>[2x]GSSSTEVKDNVLTEEEKAEGYTLLFNGKDFT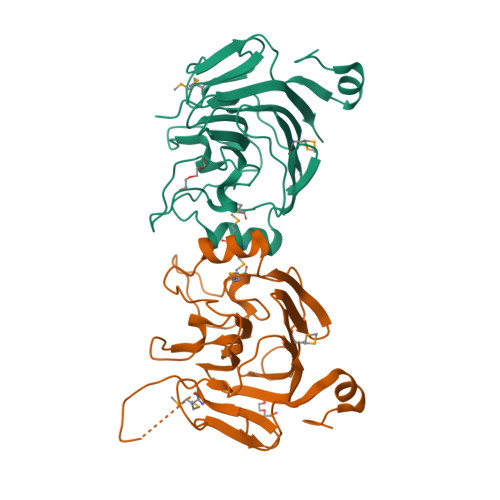GWKMFNGGDVKGWQVEDGVIVGYGNGGDVIADTTIKVSTDIVTVKNYHNFQIKWDWKIGAQGNSGFLYHVQEGPKYKAPFETGPEYQLIDDDNYPWVSETGKEGLEDWQKTGCNYAMYVPETKQVNPPGEWNSSMVLYKDGYVEHWLNGEKLFSFQEGSEDWKMRRYSGKWEAFPDYGISTTGKLCFQDHGSKVYFKNVKIKDLD>MKSGIYQIKNTLNNKVYVGSAKDFEKAWKRHFKDLEKGCHSSIKLQRSFNKHGNVFECSILEEIPYEKDLIIERENFWIKELNSKINGY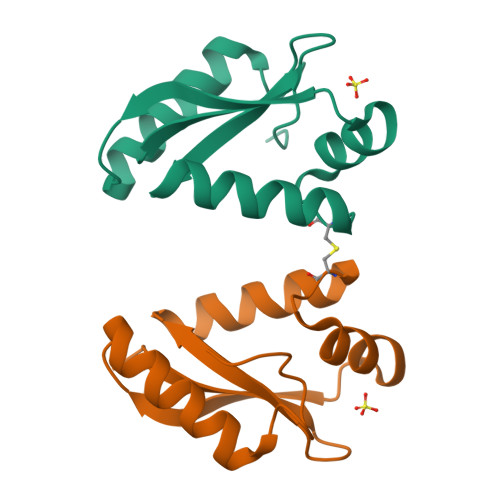NIADATFG[2x]>AHHHHHHGSEFKRLTPYEEALSIVLNDLKEIEEVEYVPLKDALGRVLAEDIVASYDLPPFDRAAVDGYAVRAEDTFEAREYSPVELEVIEEVPIGENPNKEVIAGKAIKVLTGGKIPRGANAVIMQEMVKREGSKIYVLRPVAPGQNISFAGEDVKKGDIALKKGTILRPQDLALLKALGIRKVPVKVKPKVGIIITGSELVQEPSLEEFEKGKIVDTNSIMLSALVERYFGEPILYGVVPDNEDLIRSALEKAKRECDLVLITGGSAFGDMDYAHKFVNL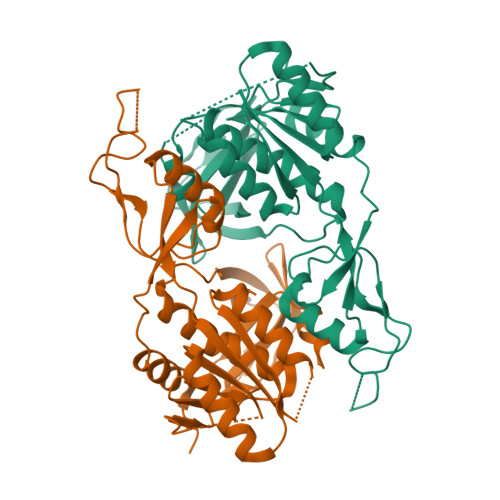LFHGTTIRPGRPIGYGERVFVMSGYPVAVFTQFHLFVKHALAKLVGAKDYEVKVRAVLEDDVPSQLGRYEFVRVMYRDGKAKVIKKKGSGIISSLVQSNAYLVVPEDVEGYRRGEEVWVTLY[2x]>QSIKWQPHQQNKWATLYDANYKELPMLTYRVDADKGFNFSVGDDAFVCQKKNHFQVTVYIGMLGEPKYVKTPEGLKPLDCFYLKLHGVKLEALNQSINIEQSQSDRSKRPFNPVTVNLPPEQVTKVTVGRLHFSETTANNMRKKGKPN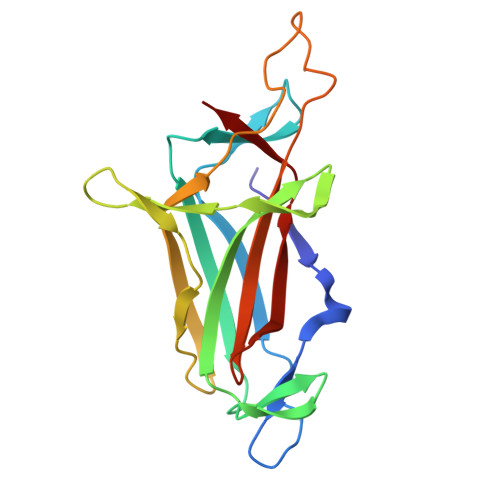PDQRYFMLVVALQAHAQNQNYTLAAQISERIIVRA[3x]> GAMADDEKNALPISKDGYIRVPKERVNVNLTSIKKLREKVDDSIHRELTDIFANLNYVGVVDEERRLAAIQHDLKLFLIDYGSVCYELFYQIGLTDFANFGKINLQSTNVSDDIVLYNLLSEFDELNDDASKEKIISKIWDMSSMLNEYYSIELVNDGLDNDLKSVKLKSLPLLLKGYIPSLVKLPFFIYRLGKEVDWEDEQECLDGILREIALLYIPDMVPKVDTSDASLSEDEKAQFINRKEHISSLLEHVLFPCIKRRFLAPRHILKDVVEIANLPDLYKVFERC;> GSKRKSEAQENIIKNKDELEDFEQGEKYLTLTVSKNDFKKMEVVGQFNLGFIIVTRKVDNKYDLFIVDQHASDEKYNFETLQAVTVFKSQKLIIPQPVELSVIDELVVLDNLPVFEKNGFKLKIDEEEEFGSRVKLLSLPTSKQTL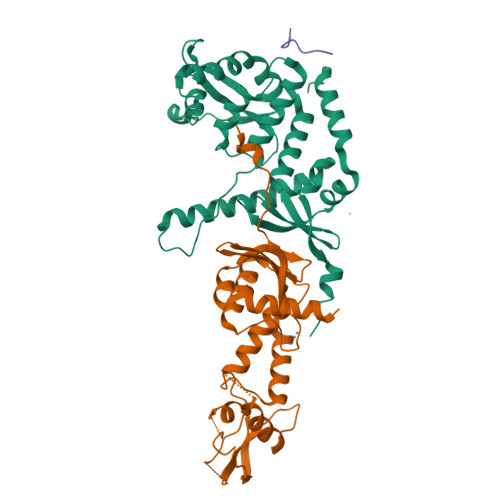FDLGDFNELIHLIKEDGGLRRDNIRCSKIRSMFAMRACRSSIMIGKPLNKKTMTRVVHNLSELDKPWNCPHGRPTMRHLMELRDWSSFSKDYEI;> TRSKFFNK>[4x]MIVILDNGGQYVHRIHRSLKYIGVSSKIVPNTT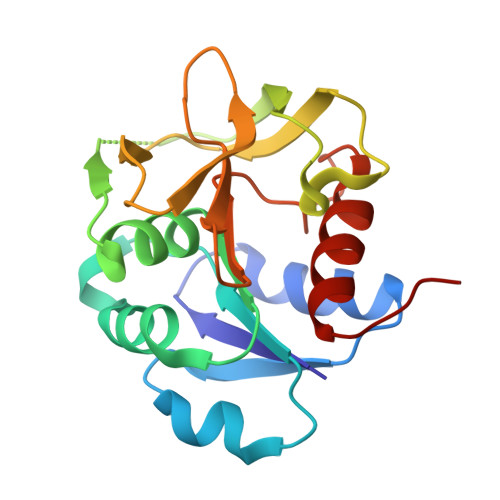PLEEIESNKEVKGIILSGGPDIEKAKNCIDIALNAKLPILGICLGHQLIALAYGGEVGRAEAEEYALTKVYVDKEPDLFKNVPREFNAWASHKDEVKKVPEGFEILAHSDICQVEAMKHKTKPIYGVQFHPEVAHTEYGNEILKNFCKVCGYKFE> MAAPTPARPVLTHLLVALFGMGSWAAVNGIWVELPVVVKELPEGWSLPSYVSVLVALGNLGLLVVTLWRRLAPGKDEQVPIRVVQVLGMVGTALLASLWHHVAPVAGQLHSVAFLALAFVLALACCASNVTFLPFLSHLPPRFLRSFFLGQGLSALLPCVLALVQGVGRLECPPAPINGTPGPPLDFLERFPASTFFWALTALLVASAAAFQGLLLLLPPPPSVPTGELGSGLQVGAPGAEEEVEESSPLQEPPSQAAGTTPGPDPKAYQLLSARSACLLGLLAATNALTNGVLPAVQSFSCL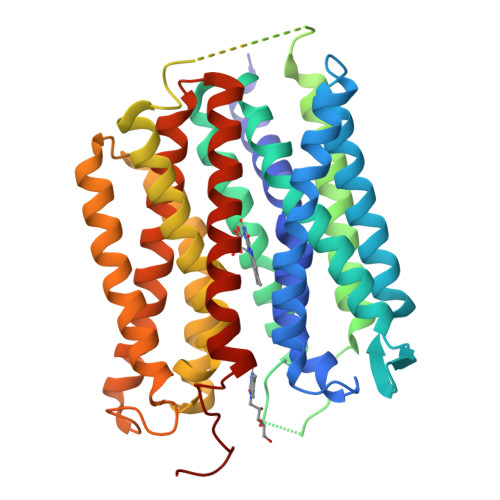PYGRLAYHLAVVLGSAANPLACFLAMGVLCRSLAGLGGLSLLGVFCGGYLMALAVLSPCPPLVGTSAGVVLVVLSWVLCLGVFSYVKVAASSLLHGGGRPALLAAGVAIQVGSLLGAVAMFPPTSIYHVFHSRKDCADPCDS Transcription termination is an essential step in transcription by RNA polymerase (RNAP) and crucial for gene regulation. For many bacterial genes, transcription termination is mediated by the adenosine triphosphate–dependent RNA translocase/helicase Rho, which causes RNA/DNA dissociation from the RNAP elongation complex (EC). Rho is an adenosine triphosphate (ATP)–dependent RNA translocase/helicase with 5′ → 3′ directionality. Rho forms a ring-shaped homo-hexameric complex, mediated by the CTD.

Cryo-EM maps of Rho, apo RNAP, EC, and type 1 and type 2 complexes are shown. When the apo RNAP structure is superimposed with the Rho-engaged EC structure, the opened clamp in apo RNAP fits with the bottom parts of the Rho hexamer without severe steric clash (protomers E and F).

>[2x]MLDSKLKAPVFTVRTQGREYGEFVLEPLERGFGVTLGNPLRRILLSSIPGTAVTSVYIEDVLHEFSTIPGVKEDVVEIILNLKELVVRFLNPSLQTVTLLLKAEGPKEVKARDFLPVADVEIMNPDLHIATLEEGGRLNMEVRVDRGVGYVPAEKHGIKDRINAIPVDAVFSPVRRVAFQVEDTRLGQRTDLDKLTLRIWTDGSVTPLEALNQAVEILREHLTYFSNPQAAAVAAPEEAKEPEAPPEQEEELDLPLEELGLSTRVLHSLKEEGIESVRALLALNLKDLKNIPGIGERSLEEIKEALEKKGFTLKE;> MEIKRFGRIREVIPLPPLTEIQVESYRRALQADVPPEKRENVGIQAAFRETFPIEEEDKGKGGLVLDFLEYRLGEPPFPQDECREKDLTYQAPLYARLQLIHKDTGLIKEDEVFLGHIPLMTEDGSFIINGADRVIVSQIHRSPGVYFTPDPARPGRYIASIIPLPKRGPWIDLEVEPNGVVSMKVNKRKFPLVLLLRVLGYDQETLARELGAYGELVQGLMDESVFAMRPEEALIRLFTLLRPGDPPKRDKAVAYVYGLIADPRRYDLGEAGRYKAEEKLGIRLSGRTLARFEDGEFKDEVFLPTLRYLFALTAGVPGHEVDDIDHLGNRRIRTVGELMTDQFRVGLARLARGVRERMLMGSEDSLTPAKLVNSRPLEAAIREFFSRSQLSQFKDETNPLSSLRHKRRISALGPGGLTRERAGFDVRDVHRTHYGRICPVETPEGANIGLITSLAAYARVDELGFIRTPYRRVVGGVVTDEVVYMTATEEDRYTIAQANTPLEGNRIAAERVVARRKGEPVIVSPEEVEFMDVSPKQVFSVNTNLIPFLEHDDANRALMGSNMQTQAVPLIRAQAPVVMTGLEERVVRDSLAALYAEEDGEVAKVDGNRIVVRYEDGRLVEYPLRRFYRSNQGTALDQRPRVVVGQRVRKGDLLADGPASENGFLALGQNVLVAIMPFDGYNFEDAIVISEELLKRDFYTSIHIERYEIEARDTKLGPERITRDIPHLSEAALRDLDEEGVVRIGAEVKPGDILVGRTSFKGESEPTPEERLLRSIFGEKARDVKDTSLRVPPGEGGIVVRTVRLRRGDPGVELKPGVREVVRVYVAQKRKLQVGDKLANRHGNKGVVAKILPVEDMPHLPDGTPVDVILNPLGVPSRMNLGQILETHLGLAGYFLGQRYISPIFDGAKEPEIKELLAQAFEVYFGKRKGEGFGVDKREVEVLRRAEKLGLVTPGKTPEEQLKELFLQGKVVLYDGRTGEPIEGPIVVGQMFIMKLYHMVEDKMHARSTGPYSLITQQPLGGKAQFGGQRFGEMEVWALEAYGAAHTLQEMLTLKSDDIEGRNAAYEAIIKGEDVPEPSVPESFRVLVKELQALALDVQTLDEKDNPVDIFEGLASKR;> MKKEVRKVRIALASPEKIRSWSYGEVEKPETINYRTLKPERDGLFDERIFGPIKDYECACGKYKRQRFEGKVCERCGVEVTKSIVRRYRMGHIELATPAAHIWFVKDVPSKIGTLLDLSATELEQVLYFSKYIVLDPKGAILNGVPVEKRQLLTDEEYRELRYGKQETYPLPPGVDALVKDGEEVVKGQELAPGVVSRLDGVALYRFPRRVRVEYVKKERAGLRLPLAAWVEKEAYKPGEILAELPEPYLFRAEEEGVVELKELEEGAFLVLRREDEPVATYFLPVGMTPLVVHGEIVEKGQPLAEAKGLLRMPRQVRAAQVEAEEEGETVYLTLFLEWTEPKDYRVQPHMNVVVPEGARVEAGDKIVAAIDPEEEVIAEAEGVVHLHEPASILVVKARVYPFEDDVEVSTGDRVAPGDVLADGGKVKSDVYGRVEVDLVRNVVRVVESYDIDARMGAEAIQQLLKELDLEALEKELLEEMKHPSRARRAKARKRLEVVRAFLDSGNRPEWMILEAVPVLPPDLRPMVQVDGGRFATSDLNDLYRRLINRNNRLKKLLAQGAPEIIIRNEKRMLQEAVDALLDNGRRGAPVTNPGSDRPLRSLTDILSGKQGRFRQNLLGKRVDYSGRSVIVVGPQLKLHQCGLPKRMALELFKPFLLKKMEEKGIAPNVKAARRMLERQRDIKDEVWDALEEVIHGKVVLLNRAPTLHRLGIQAFQPVLVEGQSIQLHPLVCEAFNADFDGDQMAVHVPLSSFAQAEARIQMLSAHNLLSPASGEPLAKPSRDIILGLYYITQVRKEKKGAGLEFATPEEALAAHERGEVALNAPIKVAGRETSVGRLKYVFANPDEALLAVAHGIVDLQDVVTVRYMGKRLETSPGRILFARIVAEAVEDEKVAWELIQLDVPQEKNSLKDLVYQAFLRLGMEKTARLLDALKYYGFTFSTTSGITIGIDDAVIPEEKKQYLEEADRKLLQIEQAYEMGFLTDRERYDQILQLWTETTEKVTQAVFKNFEENYPFNPLYVMAQSGARGNPQQIRQLCGLRGLMQKPSGETFEVPVRSSFREGLTVLEYFISSHGARKGGADTALRTADSGYLTRKLVDVTHEIVVREADCGTTNYISVPLFQPDEVTRSLRLRKRADIEAGLYGRVLAREVEVLGVRLEEGRYLSMDDVHLLIKAAEAGEIQEVPVRSPLTCQTRYGVCQKCYGYDLSMARPVSIGEAVGIVAAQSIGEPGTQLTMRTFHTGGVAGAADITQGLPRVIELFEARRPKAKAVISEIDGVVRIEETEEKLSVFVESEGFSKEYKLPKEARLLVKDGDYVEAGQPLTRGAIDPHQLLEAKGPEAVERYLVEEIQKVYRAQGVKLHDKHIEIVVRQMMKYVEVTDPGDSRLLEGQVLEKWDVEALNERLIAEGKTPVAWKPLLMGVTKSALSTKSWLSAASFQNTTHVLTEAAIAGKKDELIGLKENVILGRLIPAGTGSDFVRFTQVVDQKTLKAIEEARKEAVEAKERPAARRGVKREQPGKQADYKDDDDK;> MAEPGIDKLFGMVDSKYRLTVVVAKRAQQLLRHGFKNTVLEPEERPKMQTLEGLFDDPNAVTWAMKELLTGRLVFGENLVPEDRLQKEMERLYPGEREE> MTSFAPTVKICENLSQMSFAAREVILAAIDARVDKSVPVVLALSGGSTPKRLYEELHEKDLALLQQHAVQFILGDERLLSEDDEQSNFSMATK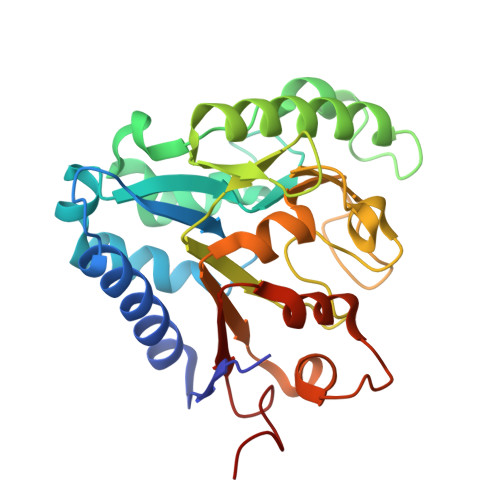ALLRDVPSSDVISIDRRAALATSKDEKGGLDGAWAVAQDYEVKLLNCLPCKQINGTAKSVPVVDIVLLGFGSDGHTASIFPDSVAATDEEHVVSVSFPSPTMSPKVWRVTLSKTVIQYAKHVVVLAAGKDKNWVVRGVLSESPTDPLPVSRFLRDCRGSVTLLLDPGAGEGVCA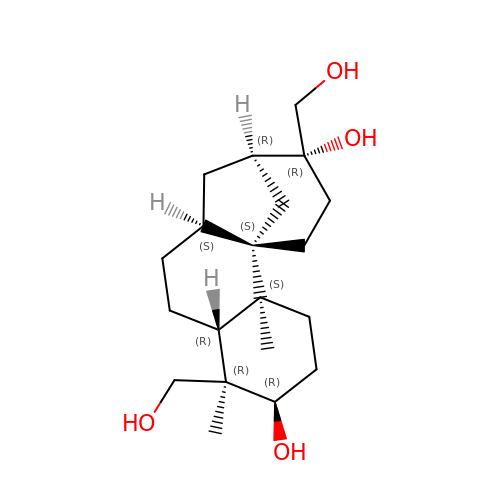(3R,4R,4aR,6aS,8R,9R,11aS,11bS)-4,9-bis(hydroxymethyl)-4,11b-dimethyltetradecahydro-8,11a-methanocyclohepta[a]naphthalene-3,9-diol | C20 H34 O4 | NOFOAYPPHIUXJR-APNQCZIXSA-N> 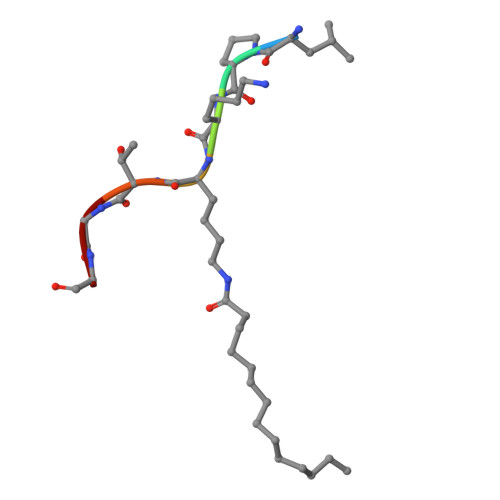LPKXTGG> LEPRHAMLLRCRLPGGVITTKQ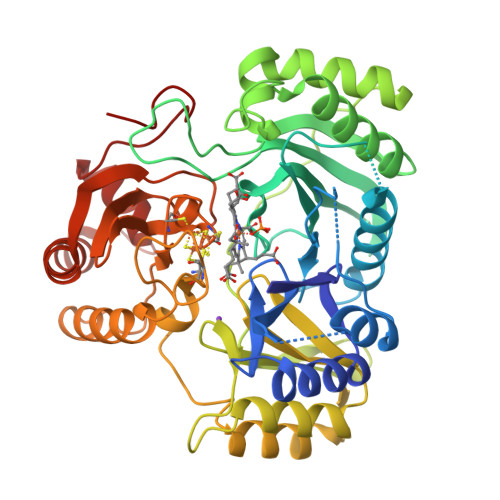WQAIDKFAGENTIYGSIRLTNRQTFQFHGILKKNVKPVHQMLHSVGLDALATANDMNRNVLCTSNPYESQLHAEAYEWAKKISEHLLPRTRAYAEIWLDQEKVATTDEEPILGQTYLPRKFKTTVVIPPQNDIDLHANDMNFVAIAENGKLVGFNLLVGGGLSIEHGNKKTYARTASEFGYLPLEHTLAVAEAVVTTQRDWGNRTDRKNAKTKYTLERVGVETFKAEVERRAGIKFEPIRPYEFTGRGDRIGWVKGIDDNWHLTLFIENGRILDYPARPLKTGLLEIAKIHKGDFRITANQNLIIAGVPESEKAKIEKIAKESGLMNAVTPQRENSMACVSFPTCPLAMAEAERFLPSFIDNIDNLMAKHGVSDEHIVMRVTGCPNGCGRAMLAEVGLVGKAPGRYNLHLGGNRIGTRIPRMYKENITEPEILASLDELIGRWAKEREAGEGFGDFTVRAGIIRPVLDPARDLWD>WGNLGHETVAYIAQSFVASSTESFCQNILGDDSTSYLANVATWANTYKYTDAGEFSKPYHFIDAQDNPPQSCGVDYDRDCGSAGC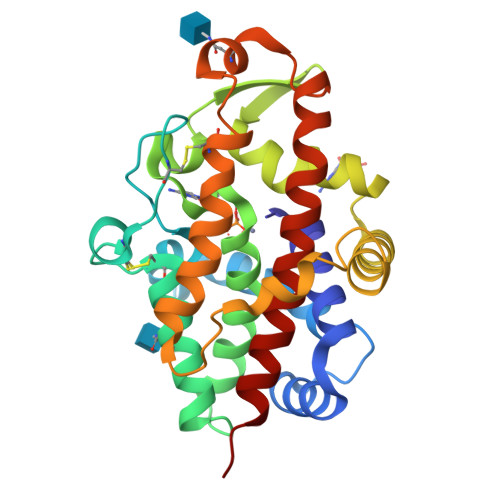SISAIQNYTNILLESPNGSEALNALKFVVHIIGDIHQPLHDENLEAGGNGIDVTYDGETTNLHHIWDTNMPEEAAGGYSLSVAKTYADLLTERIKTGTYSSKKDSWTDGIDIKDPVSTSMIWAADANTYVCSTVLDDGLAYINSTDLSGEYYDKSQPVFEELIAKAGYRLAAWLDLIASQPS[2x]>[4x]GSHMSAPLPLDELRTFAEVLDRVKAAYVEPVDDKTLLENAIKGMLSNLDPHS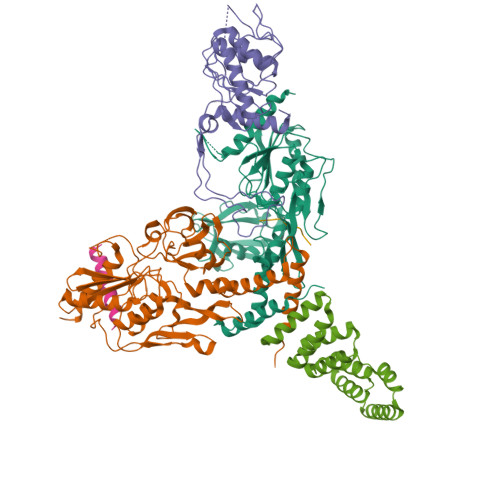AYLGPEDFAELQESTSGEFGGLGIEVGSEDGFIKVVSPIDDTPAARAGIQPGDLIVQIDGKPTKGQSMTEAVDSMRGKAGSPITLTIVRDGGRPFDVELKRAIIKVKSVKSQVLEPGYAYLRITQFQVNTGEEVVKALNQLRKDNKGRLKGLVLDLRNNPGGVLQSAVEVADAFLTKGLIVYTKGRIANSELRFSADPADPSDKVPLVVLINGGSAAAAEIVAGALQDQKRAILMGTDSFGKGSVQTVLPLNNDRALKLTTALYYTPNGRSIQAQGIVPDIEVGRAKVTQERSSFEGFKEADLQGHLANGNGGADRPTGKRAAPSERPQDSDYQLSQALSLLKGLSVTRGN;> MEDTAVETKAKPEKYGSFSEDSLYSLLVAELAGQRNRFDIALSNYVVQAQKTRDPGVSERAFRIAEYLGADQEALDTSLLWARSAPDNLDAQRAAAIQLARAGRYEESMVYMEKVLNGQGDTHFDFLALSAAETDPDTRAGLLQSFDHLLKKYPNNGQLLFGKALLLQQDGRPDEALTLLEDNSASRHEVAPLLLRSRLLQSMKRSDEALPLLKAGIKEHPDDKRVRLAYARLLVEQNRLDDAKAEFAGLVQQFPDDDDLRFSLALVCLEAQAWDEARIYLEELVERDSHVDAAHFNLGRLAEEQKDTARALDEYAQVGPGNDFLPAQLRQTDVLLKAGRVDEAAQRLDKARSEQPDYAIQLYLIEAEALSNNDQQEKAWQAIQEGLKQYPEDLNLLYTRSMLAEKRNDLAQMEKDLRFVIAREPDNAMALNALGYTLADRTTRYGEARELILKAHKLNPDDPAILDSMGWINYRQGKLADAERYLRQALQRYPDHEVAAHLGEVLWAQGRQGDARAIWREYLDKQPDSDVLRRTIKRLTGAETP> HMGRSQNSEFETASDEPIAVIGLSCRLPKASGPQELWQLLDDGASAVTRVPADRETPPSTEEESADGEAAGARWGGFLDRVDTFDAGFFGISPREAAAMDPQQRLVLELSWEALEGAGLVPATLRDTGLGVFVGAARDDYATLYRRREGRAVDHHAMTGLHRSLIANRISYALGAHGPSMVVDTGCSSSLVAVHLACESLRRGESDIALAGGVNLNIAAESARETAAFGGLSPDGQCFTFDARANGFVRGEGGGLVVLKTLRRALADGDLVHGVILASAVNNDGPSDTLTTPSRRAQESLLTRVYRRAGVTPTEVGYVELHGTGTKVGDPIEAAALGAVLGTGRDTPLPVGSIKTNIGHLEGAAGIAGLIKALLQLRRRRLVPSLNFSTPNPDIPLDALNLRVQQESAPWATPSGGGRTLVAGVSSFGMGGTNCHVVVSAAPVPEDGETTSEAGATGPDSGPALLPWVVSARSPQALRDQAGRLAAWADSPAGREASPVDIGWSLATSRTHFEYRAVVSGSDRDELVASLRALASGSPVTAAGAVDGGGRLGLVFSGQGSQRAGMGREL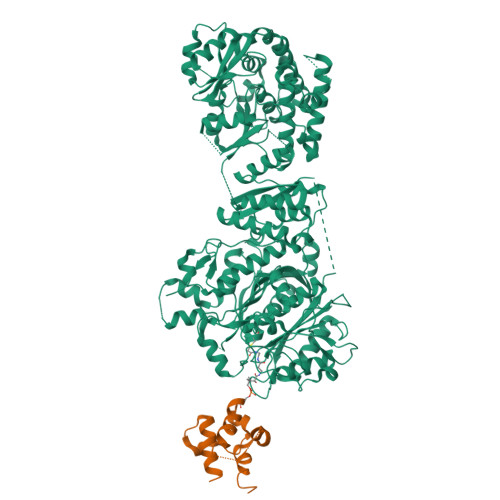YVAFPVFAEAFDEVCGVLDEVMGALPPSEGWAGSLREVMFEVSSDLLDETGFTQPALFAFEVALYRLLESWGVAGEVVAGHSVGEIAAVHVAGVLSLADACALVAARGRLMQGLPSGGAMVAVEASEEEVTALLAGREGEVGIGAVNGPRSVVVSGGVAVVEEVAAHFAGLGRRARRLKVSHAFHSPLMDPMLEDFGRVVAGLSFAVPELTVVSGLTGAVVSADELCSVGYWVRHAREAVRFADAVGAMAGVGVGRFVEVGPGGVLSALVRECLAEGGAGSVVAAVRGNRAEPVALLSAVGELFADGYPVDWTAYFAGWPAARVELPTYAFQRSRHWLENVPELAVS;> HMPREPVTPDSDHPDPVETVRQLTAHVLGLTAAADVEMTRSFKDLGFDSLMSVELRDRLCAATGLSLATTLLYDHPSPAETAEFVRARLTGDEA> MASMTGGQQMGRGSMIFSVDKVRADFPVLSREVNGLPLA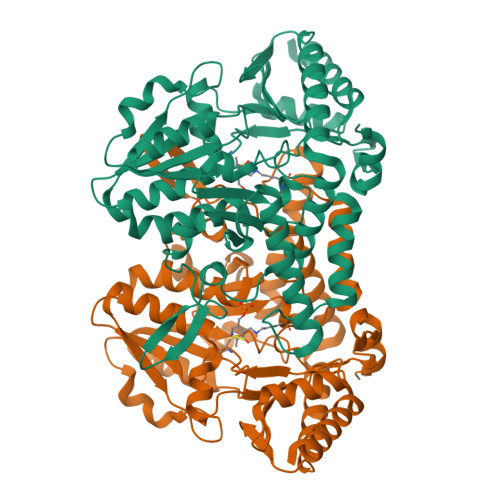YLDSAASAQKPSQVIDAEAEFYRHGYAAVARGIHTLSAQATEKMENVRKRASLFINARSAEELVFVRGTTEGINLVANSWGNSNVRAGDNIIISQMEHHANIVPWQMLCARVGAELRVIPLNPDGTLQLETLPTLFDEKTRLLAITHVSNVLGTENPLAEMITLAHQHGAKVLVDGAQAVMHHPVDVQALDCDFYVFSGHKLYGPTGIGILYVKEALLQEMPPWEGGGSMIATVSLSEGTTWTKAPWRFEAGTPNTGGIIGLGAALEYVSALGLNNIAEYEQNLMHYALSQLESVPDLTLYGPQNRLGVIAFNLGKHHAYDVGSFLDNYGIAVRTGHHCAMPLMAYYNVPAMCRASLAMYNTHEEVDRLVTGLQRIHRLLG> MLRAKVRRIALANQKGGVGKTTTAINLAAYLARLGKRVLLVDLDPQGNATSGLGVRAERGVYHLLQGEPLEGLVHPVDGFHLLPATPDLVGATVELAGAPTALREALRDEGYDLVLLDAPPSLSPLTLNALAAAEGVVVPVQAEYYALEGVAGLLATLEEVRAGLNPRLRLLGI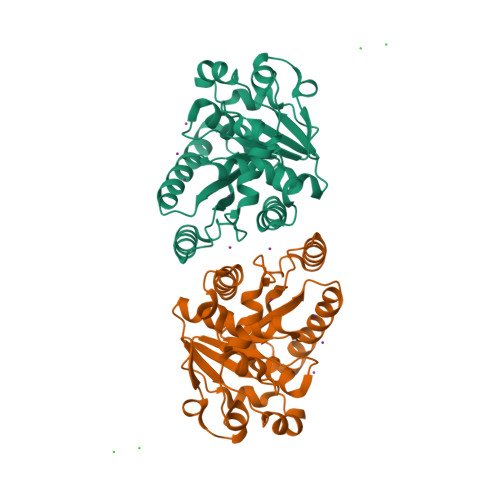LVTMYDGRTLLAQQVEAQLRAHFGEKVFWTVIPRNVRLAEAPSFGKTIAQHAPTSPGAHAYRRLAEEVMARVQEAGSHHHHHH>ATCYCRTGRCATR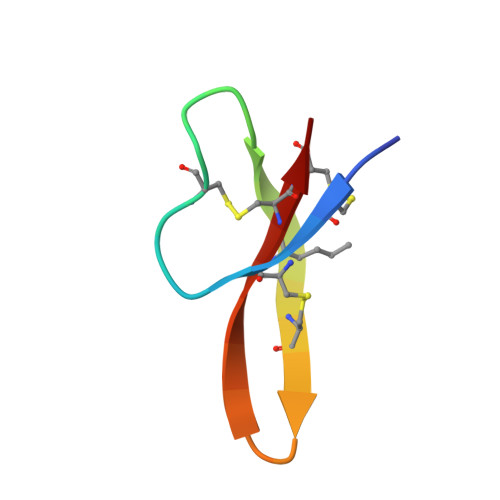ESLSGVCEISGRLYRLCCR[2x]>[6x]MMTHEENELLCRVEGDAPMGRLMRRHWTPICLVEEVGEPDGTPVKARAFGEDLVVFRDSEGRVGVMDEYCPHRRASLVYGRNEEGGLRCLYHGWKMDVDGNVLEMASEPAASGMVDKVKHTAYPTQEWAGMVWAYMGPKETMPEFLPPAWAPTADTRVSIAKVLLPCNWAQILEGAIDSAHSSSLHSSDMVPARVDGAKATDKTWLRP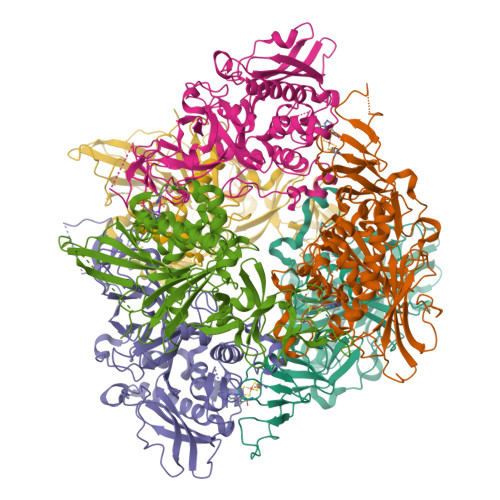STDKAPRMQVQRTGYGFRYAALRRPLSNAAENDYVRSTVFVAPATALIPPNNLYNVANINVPMDDTNTAFYFIAWGHPSQTPETETWRKFLRQTVGVDLDQNYRPLRNEANKFWQDRNAMKAGNFTGITGFPNQDVAMWLTMGPIADRTHDRLGASDLAIVEFRKQMLDAVKAFEQGAPAIGTGVEAATPTVCSFQAIVPKTTDWRTYDAHYVWLDGQDRPEFEPSYSVKS> RAGPVTWVMMIACVVVFIAMQILGDQEVMLWLAWPFDPTLKFEFWRYFTHALMHFSLMHILF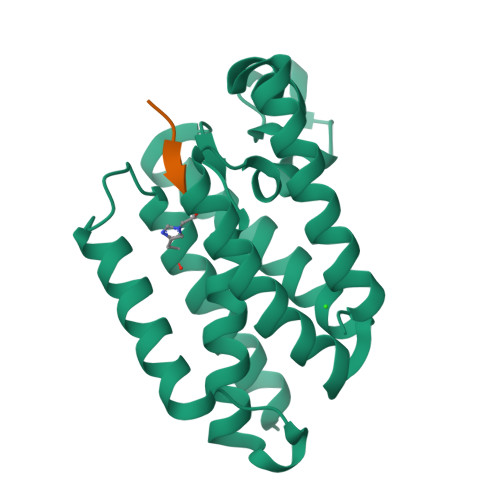NLLWWWYLGGAVEKRLGSGKLIVITLISALLSGYVQQKFSGPWFGGLSGVVYALMGYVWLRGERDPQSGIYLQRGLIIFALIWIVAGWFDLFGMSMANGAHIAGLAVGLAMAFVDSL>LTEGNPRWEQTHLRYRIENYTPDLPRADVDHAIEKAFQLWSNVTPLTFTKVSEGQADIMISFVRGDHRDNSPFDGPGGNLAHAFQPGPGIGGDAHFDEDERWTNNFREYNLHRVAAHELGHSLGLSHSTDIGALMYPSYTFSG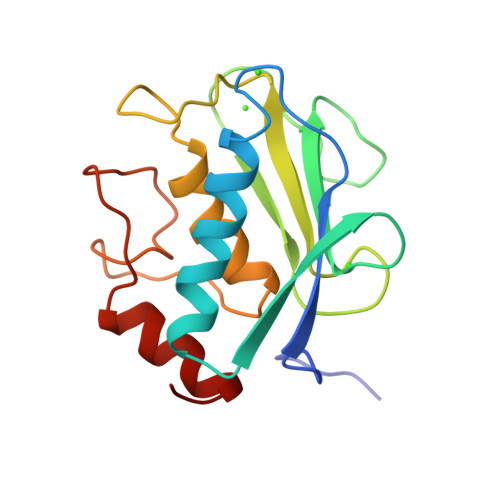DVQLAQDDIDGIQAIYGRS[2x]>MASHHHHHHHENLYFQGMSGIQTVSKSATDLTEMVKKITTMNRGEFRQITLATGAGKTTELPRSVIEEIGRHKRVLVLIPLRAAAESVYQYMRQKHPSIAFNLRIGEMKEGDMATGITYASYGYFCQMSQPKLRAAMVEYSFIFLDEYHCATPEQLAIMGK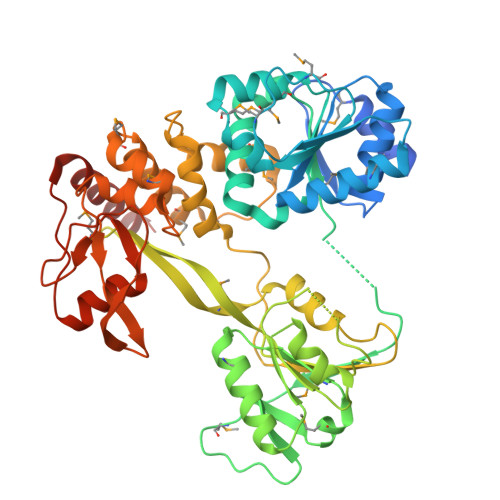IHRFSENLRVVAMTATPAGTVTTTGQKHPIEEFIAPEVMKGEDLGSEYLDIAGLKIPVEEMKNNMLVFVPTRNMAVEAAKKLKAKGYNSGYYYSGEDPSNLRVVTSQSPYVVVATNAIESGVTLPDLDVVVDTGLKCEKRIRLSPKMPFIVTGLKRMAVTIGEQAQRRGRVGRVKPGRYYRSQETPVGSKDYHYDLLQAQRYGIEDGINITKSFREMNYDWSLYEEDSLMITQLEILNNLLISEELPMAVKNIMARTDHPEPIQLAYNSYETQVPVLFPKIRNGEVTDTYDNYTFLNARKLGDDVPPYVYATEDEDLAVELLGLDWPDPGNQGTVEAGRALKQVVGLSTAENALL[4x]>[2x]MANELTWHDVLAEEKQQPYFLNTLQTVASERQSGVTIYPPQKDVFNAFRFTELGDVKVVILGQDPYHGPGQAHGLAFSVRPGIAIPPSLLNMYKELENTIPGFTRPNHGYLESWARQGVLLLNTVLTVRAGQAHSHASLGWETFTDKVISLINQHREGVVFLLWGSHAQKKGAIIDKQRH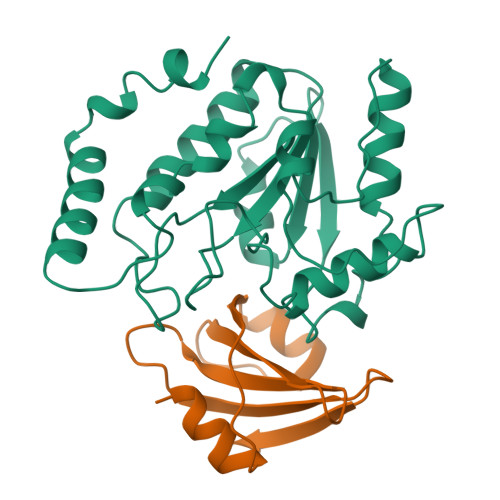HVLKAPHPSPLSAHRGFFGCNHFVLANQWLEQRGETPIDWMPVLPAESE;>MTNLSDIIEKETGKQLVIQESILMLPEEVEEVIGNKPESDILVHTAYDESTDENVMLLTSDAPEYKPWALVIQDSNGENKIKML[2x]> ADFDAVLKCWGPVEADYTTMGG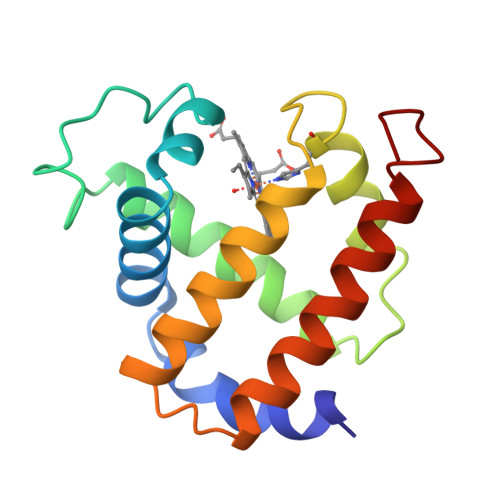LVLTRLFKEHPETQKLFPKFAGIAQADIAGNAAISAHGATVLKKLGELLKAKGSHAAILKPLANSHATKHKIPINNFKLISEVLVKVMHEKAGLDAGGQTALRNVMGIIIADLEANYKELGFSG> VVGGTDADEGEWPWQVSLHALGQGHICGASLISPNWLVSAAHCYIDDRGFRYSDPTQWTAF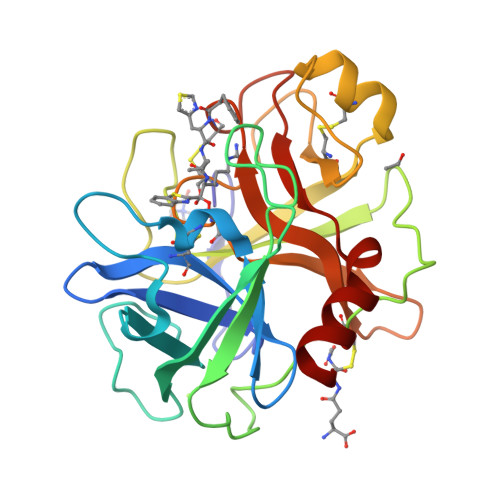LGLHDQSQRSAPGVQERRLKRIISHPFFNDFTFDYDIALLELEKPAEYSSMVRPICLPDASHVFPAGKAIWVTGWGHTQYGGTGALILQKGEIRVINQTTCENLLPQQITPRMMCVGFLSGGVDSCQGDSGGPLSSVEADGRIFQAGVVSWGDGCAQRNKPGVYTRLPLFRDWIKENTGV> SRLNRESVIDAALELLNETGIDGLTTRKLAQKLGIEQPTLYWHVKNKRALLDALAVEILARHHDYSLPAAGESWQSFLRNNAMSFRRALLRYRD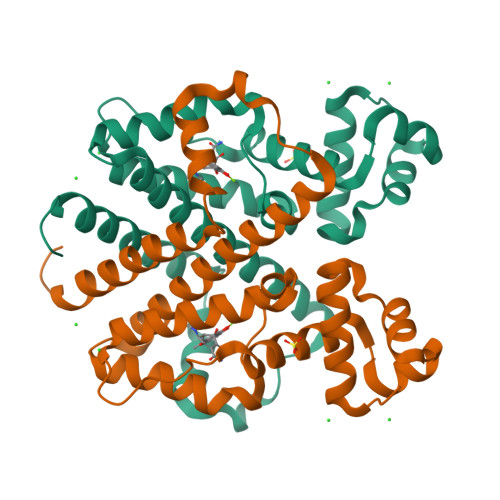GAKVHLGTRPDEKQYDTVETQLRFMTENGFSLRDGLYAISAVSHFTLGAVLEQQEHTAALTDRPAAPDENLPPLLREALQIMDSDDGEQAFLHGLESLIRGFEVQLTALLQIVGGDKLIIPFC> SADAQSFLNRVCGVSAARLTPCGTGTSTDVVYRAFDIYNDKVAGFAKFLKTNCCRFQEKDEDDNLIDSYFVVKRHTFSNYQHEETIYNLLKDCPAVAKHDFFKFRIDGDMVPHISRQRLTKYTMADLVYALRHFDEGNCDTLKEILVTYNCCDDDYFNKKDWYDFVENPDILRVYANLGERVRQALLKTVQFCDAMRNAGIVGVLTLDNQDLNGNWYDFGDFIQTTPGSGVPVVDSYYSLLMPILTLTRALTAESHVDTDLTKPYIKWDLLKYDFTEERLKLFDRYFKYWDQTYHPNCVNCLDDRCILHCANFNVLFSTVFPPTSFGPLVRKIFVDGVPFVVSTGYHFRELGVVHNQDVNLHSSRLSFKELLVYAADPAMHAASGNLLLDKRTTCFSVAALTNNVAFQTVKPGNFNKDFYDFAVSKGFFKEGSSVELKHFFFAQDGNAAISDYDYYRYNLPTMCDIRQLLFVVEVVDKYFDCYDGGCINANQVIVNNLDKSAGFPFNKWGKARLYYDSMSYEDQDALFAYTKRNVIPTITQMNLKYAISAKNRARTVAGVSICSTMTNRQFHQKLLKSIAATRGATVVIGTSKFYGGWHNMLKTVYSDVENPHLMGWDYPKCDRAMPNMLRIMASLVLARKHTTCCSLSHRFYRLANECAQVLSEMVMCGGSLYVKPGGTSSGDATTAYANSVFNICQAVTANVNALLSTDGNKIADKYVRNLQHRLYECLYRNRDVDTDFVNEFYAYLRKHFSMMILSDDAVVCFNSTYASQGLVASIKNFKSVLYYQNNVFMSEAKCWTETDLTKGPHEFCSQHTMLVKQGDDYVYLPYPDPSRILGAGCFVDDIVKTDGTLMIERFVSLAIDAYPLTKHPNQEYADVFHLYLQYIRKLHDELTGHMLDMYSVMLTNDNTSRYWEPEFYEAMYTPHTVLQ;>[2x]MGSSHHHHHHENLYFQSNAAIASEFSSLPSYAAFATAQEAYEQAVANGDSEVVLKKLKKSLNVAKSEFDRDAAMQRKLEKMADQAMTQMYKQARSEDKRAKVTSAMQTMLFTMLRKLDNDALNNIINNARDGCVPLNIIPLTTAAKLMVVIPDYNTYKNTCDGTTFTYASALWEIQQVVDADSKIVQLSEISMDNSPNLAWPLIVTALRANSAVKLQ;> SNASKMSDVKCTSVVLLSVLQQLRVESSSKLWAQCVQLHNDILLAKDTTEAFEKMVSLLSVLLSMQGAVDINKLCEEMLDNRAT

The RNA-dependent RNA polymerase (RdRp) consists of the polymerase subunit nsp12 and the accessory subunits nsp7 and nsp8 (4, 5). The RdRp is essential for replication and transcription of the viral genome and is therefore a highly promising drug target. Using RNA elongation and fluorescence polarization assays, we show that HeE1-2Tyr is a competitive inhibitor of RNA binding to SARS-CoV-2 RdRp and thereby prevents RNA extension.

We acquired cryo-EM datasets of RdRp without RNA, but in presence of 50 µM HeE1-2Tyr, as well as RdRp with 0.5% DMSO as a solvent control. To clearly separate particles with and without the extra density, we performed focused 3D classification without image alignment. This resulted in ~200,000 RdRp particles containing an extra density, which could be refined to 3.0 Å. The stack of three HeE1-2Tyr molecules binds directly into the RNA binding site of nsp12 between the finger, palm, and thumb domain. The stacking between the three HeE1-2Tyr molecules is driven by the aromatic pyridobenzothiazole moieties of the compound molecules, which are arranged on top of each other with a planar antiparallel geometry. Besides π–π interactions, HeE1-2Tyr2 and HeE1-2Tyr3 are stabilized by the formation of two hydrogen bonds (H-bond) between the oxygen of the ether group and the nitrogen of the amine group of each molecule. The carboxylate of HeE1-2Tyr1 and the guanidinium group of Arg836 are 3.3 Å apart, which suggests the formation of an ionic bond. Besides that, it is known from other protein-ligand structures that guanidinium groups of arginine residues can form relatively stable cation–π interactions with aromatic systems. Such a cation–π interaction is formed between the hydroxyphenyl moiety of HeE1-2Tyr1 and the guanidinium group of Arg555. HeE1-2Tyr3, which is the molecule furthest away from nsp12, forms a cation–π interaction with Arg858 of RdRp. Three RdRp arginine residues form an arginine bracket that stabilizes the stack of HeE1-2Tyr molecules within the RdRp RNA binding site by the formation of two cation–π and one ionic interaction. Indeed, when the RdRp–RNA and RdRp-HeE1-2Tyr structures are superimposed, a steric clash between the stack of HeE1-2Tyr molecules and the RNA becomes apparent.4-(3-fluoranylpyridin-4-yl)-~{N}-[(1~{R})-1-(3-methoxyphenyl)ethyl]piperazine-1-carboxamide 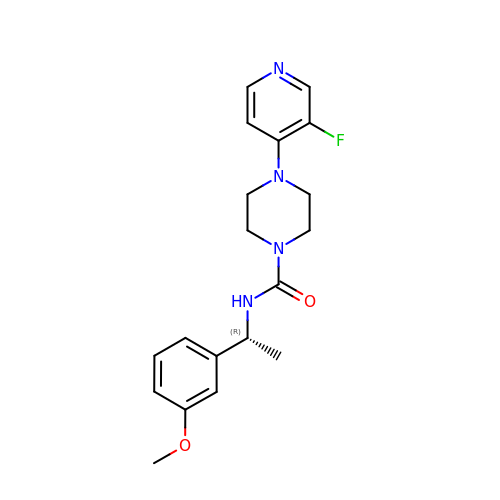| C19 H23 F N4 O2 | RLYKEFWBHJQJPK-CQSZACIVSA-N> GAGRHPPVVLVPGDLGNQLEAKLDKPTVVHYLCSKKTESYFTIWLNLELLLPVIIDCWIDNIRLVYNKTSRATQFPDGVDVRVPGFGKTFSLEFLDPSKSSVGSYFHTMVESLVGWGYTRGEDVRGAPYDWRRAPNENGPYFLALREMIEEMYQLYGGPVVLVAHSMGNMYTLYFLQRQPQAWKDKYIRAFVSLGAPWGGVAKTLRVLASGDNNRIPVIGPLKIREQQRSAVSTSWLLPYNYTWSPEKVFVQTPTINYTLRDYRKFFQDIGFEDGWLMRQDTEGLVEATMPPGVQLHCLYGTGVPTPDSFYYESFPDRDP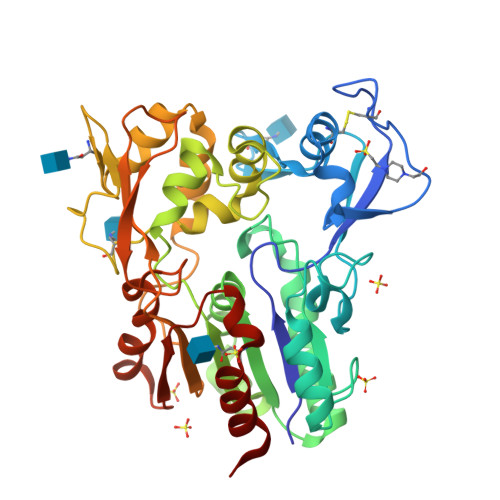KICFGDGDGTVNLKSALQCQAWQSRQEHQVLLQELPGSEHIEMLANATTLAYLKRVLLGP B. bacteriovorus is an obligate bacterial predator of other Gram-negative bacteria, exploiting adaptations that allow consumption from inside the prey cell periplasm. The DgcB protein appends the C-terminal GGDEF enzymatic domain with an N-terminal forkhead-associated (FHA) domain, known to be used (in other proteins) for interactions with phosphopeptide ligands. DgcB comprised a ~30aa tail, 100aa FHA, 20aa linker and 160aa GGDEF domain. We provide the molecular basis for initiation of c-di-GMP production, demonstrating that the stimulus is a phosphopeptide tail present on the DgcB GGDEF synthase itself.

By combining a tailless DgcB FHA construct (residues 32–131, V32 replaced with an initiating methionine) and synthetic phosphopeptide (N7SDNLEKpTSIVASDT17) in-trans, we were able to obtain complex crystals diffracting to 1.48 Å resolution. The asymmetric unit of this new form contained two FHA domains that were in an offset dimer identical to both the full-length and FHA-only structures, providing a third independent observation of this interaction. The exposed FHA cleft of chain B displays clear density for a bound phosphopeptide, allowing unequivocal modeling of residues 11–21. The conformation of the bound tail region does not differ substantially from that of the unphosphorylated complex (rmsd 1.0 Å for all atoms), but sits relatively deeper into the FHA cleft, making more extensive contacts. The more deeply situated tail is now able to form mainchain hydrogen bonds with R61, K72 and N97 (via both groups of the amide sidechain). The FHA surface creates two depressions which accommodate the two “inwardly projected” residues of the tail (pT14 and +3 V17); the flanking L11 and T21 sidechains sandwich opposing sides of the central FHA body. The central pT14 of the peptide tail is recognized by a multitude of interactions, the sidechain methyl group projecting into a pocket formed by residues 72–75 and 96–97, which positions the phosphate toward the positively charged R61 and R76. The phosphoryl group is tightly co-ordinated by the FHA cleft of DgcB: OG by R61, O1 by S95 and T96, O2 by both the backbone NH and sidechain of R76, and O3 by R76 (and the backbone NH of pT14 also). Comparison of the peptide-bound and unbound FHA domain structures reveals that peptide binding does not induce any obvious gross conformational change or long-range signaling motions, merely alterations in the rotameric states of R61, K72 and R76. Our structure of the FHA:phosphopeptide complex demonstrates that cleft occupancy does not alter the FHA:FHA contacts, at least for a peptide added in trans.

>MPPAIVVLIGPPGYVGKQYPITASDIVIGRSVESQVYIDDKSLSRSHAKFAVNGSEVSVIDLGSTNKTIVNGQVIPPLASCLLKNNDQIKTGNVIFKFLEKGS[2x];> LEKTSIVASDTX> MEPHSLRYNLTVLSWDGSVQSGFLTEVHLDGQPFLRCDRQKCRAKPQGQW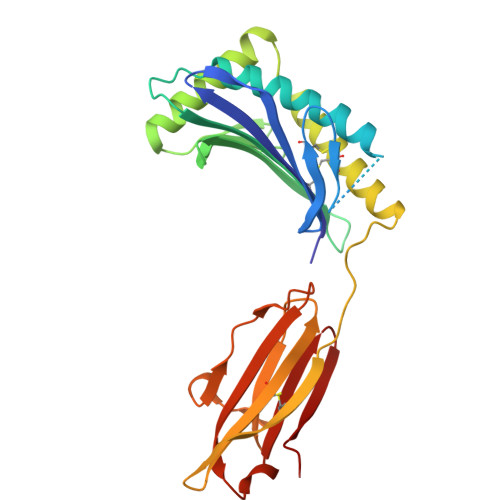AEDVLGNKTWDRETRDLTGNGKDLRMTLAHIKDQKEGLHSLQEIRVCEIHEDNSTRSSHHFYYDGELFLSWNLETKEFTMPQSSRAQTLAMNVRNFWKEDAMKTKTHFHAMHADCLQELRRYLKSGVVLRRTVPPMVNVTRSEASEGNITVTCRASGFYPWNITLSWRQDGVSLSHDTQQWGDVLPDGNGTYQTWVATRICQGEEQRFTCYMEHSGNHSTHPVPS>[5x]SMDGSRRSGYITIGYRGSYTIGRDAQADAKFRRVARITV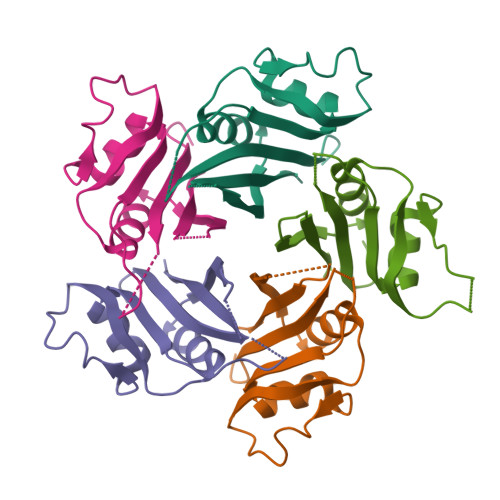CGKTSLAKEVFGDTLNESRDPDRPPERYTSRYYLKFNFLEQAFDKLSESGFHMVACSSTGTCAFASSTDQSEDKIWTSYTEYVFCRE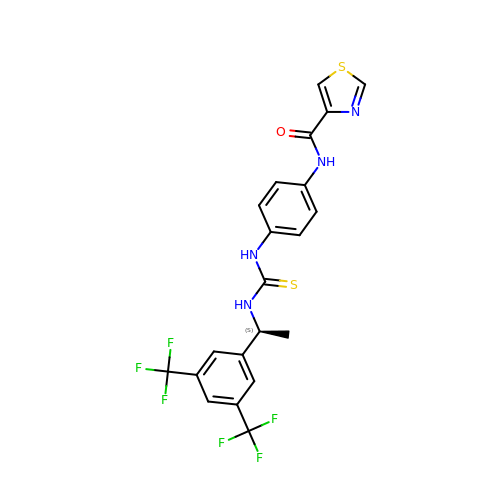N-{4-[({(1S)-1-[3,5-bis(trifluoromethyl)phenyl]ethyl}carbamothioyl)amino]phenyl}-1,3-thiazole-4-carboxamide | C21 H16 F6 N4 O S2 | NKTPIWMJHDVAPY-NSHDSACASA-N>[3x]GGCGACCCUGAUGAGGCC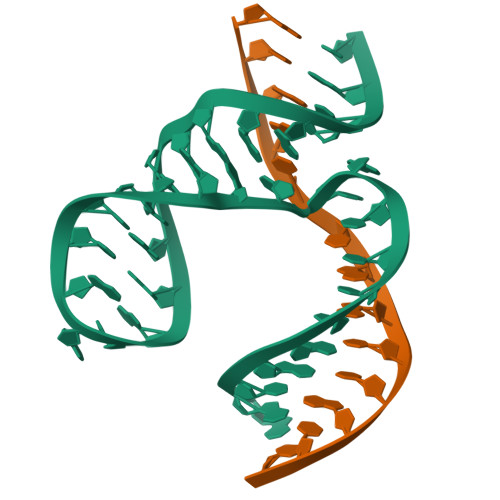GAAAGGCCGAAACCGU;>ACGGTCGGTCGCC[3x]>[2x]MNISSAQFIPGVHTVEEIEAEIHKNLHISKSCSYQKVPNSHKEFTKFCYEVYNEIKISDKEFKEKRAALDTLRLCL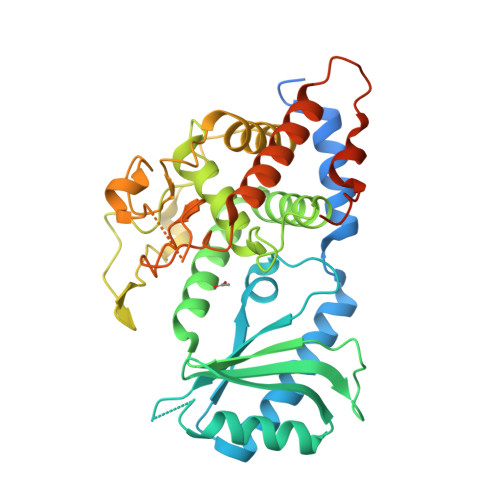KRISPDAELVAFGSLESGLALKNSDMDLCVLMDSRVQSDTIALQFYEELIAEGFEGKFLQRARIPIIKLTSDTKNGFGASFQCDIGFNNRLAIHNTLLLSSYTKLDARLKPMVLLVKHWAKRKQINSPYFGTLSSYGYVLMVLYYLIHVIKPPVFPNLLLSPLKQEKIVDGFDVGFDDKLEDIPPSQNYSSLGSLLHGFFRFYAYKFEPREKVVTFRRPDGYLTKQEKGWTSATEHTGSADQIIKDRYILAIEDPFEISHNVGRTVSSSGLYRIRGEFMAASRLLNSRSYPIPYDSLFEEAPIPPRRQKKTDEQSNKKLLNETDGDNSE> GPPPGPPRVSPDPRAELDSTVLLTRSLLADTRQLAAQLRDKFPADGDHNLDSLPTLAMSAGALGALQLPGVLTRLRADLLSYLRHVQWLRRAGGSSLKTLEPELGTLQARLDRLLRRLQLLMSRLALPQPPPDPPAPPLAPP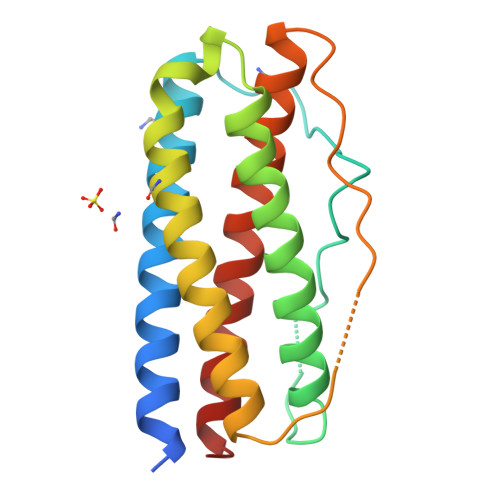SSAWGGIRAAHAILGGLHLTLDWAVRGLLLLKTRL> GPISEFPVDFHYGVRVDVTLLSKIRRVNEHIKSATKTGVVQVHGSACTPTLSVLSSVGTAGVLGMRIKNALTPLVGHTEGSGDVSFSFRNTSVGSGFTHTRELFGANVLDAGIAFYRKGEACDTGAQPQFVRTTISYGDNLTSTVHKSVVDQKGILPFHDRMEAGGRTTRLMLCGKTG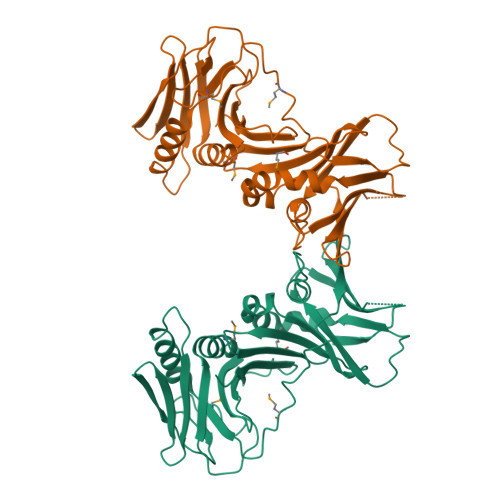AFLLKWLRQQKTKEDQTVTVSVSETLSIVTFSLGGVSKIIDFKPETKPVSGWDGLKGKKSVDVGVVHTDALSRVSLESLIAALRMCKVPGWFTPGLIWHSNEILEVEGVPTGCQSGDVKLSVLLLEVNRSV The FAD-dependent oxidoreductase from Chaetomium thermophilum (CtFDO) is a novel thermostable glycoprotein from the glucose–methanol–choline (GMC) oxidoreductase superfamily. However, CtFDO shows no activity toward the typical substrates of the family and high-throughput screening with around 1000 compounds did not yield any strongly reacting substrate. The structure of CtFDO reveals an unusually wide-open solvent-accessible active-site pocket with a unique His–Ser amino-acid pair putatively involved in enzyme catalysis. A series of six crystal structures of CtFDO complexes revealed five different subsites for the binding of aryl moieties inside the active-site pocket and conformational flexibility of the interacting amino acids when adapting to a particular ligand.

Cystamine, which was used for CtFDO complex preparation by co-crystallization, was found to improve the diffraction quality of the CtFDOdegl crystal, but without any electron density being found for the compound. The structure is presented as the ligand-free structure of CtFDOdegl and is referred to as the CtFDO:free structure. The CtFDO:free crystal structure has two CtFDOdegl molecules (chains A and B) in the asymmetric unit, with an r.m.s.d. on Cα atoms of 0.12 Å. The cofactor is noncovalently bound to the apo­enzyme via hydrogen bonds to 13 surrounding residues (Ile56, Ser57, Glu77, Ala78, Val124, Gly128, Asn132, Ala133, Val135, Val273, Ile597, Ser607 and Met609) and indirectly via 12 water molecules. A composite OMIT map of the isoalloxazine ring confirms the nonplanar conformation of the ring with a 20.0° (21.4° in chain B) bend around the N5–N10 axis (measured for atoms C4—N5—C6), which indicates the reduced state of the cofactor. Absorption spectra of an unliganded CtFDOdegl crystal measured before and after X-ray exposure showed that FAD was oxidized before and reduced after exposure and that the reduction occurred during X-ray exposure. One exception is His564, which is always modelled in one conformation enforced by the stabilizing hydrogen bond with Gln351. The active-site pocket of CtFDO:free is occupied by water molecules, two of which are in the CS. The first one, the active-site water molecule (WAS), was found bridging four atoms: His564 Nɛ2 (3.0 Å; 3.1 Å in chain B), Ser607 Oγ (‘in’ conformer, 3.1 Å; 2.9 Å in chain B), Asn562 Nδ2 (3.3 Å) and FAD O4 (3.5 Å). The second water molecule, which is more distant from the isoalloxazine ring (WDAS), is bound between WAS (2.4 Å; 2.6 Å in chain B), Asn562 Nδ2 (3.5 Å; 3.4 Å in chain B), FAD O4 (3.6 Å; 3.8 Å in chain B) and Tyr OH (3.5 Å in chain B, 4.7 Å in chain A).

>NVHSNYTFIIAGGGISGLTLADRLTEDPRVTVLVIEAGPLDRGEDGILVPGAFSPWLYFWPGLVSTPQAGLNNRTVDVITAQVVGGGSTINAMVYLRGDKDDYDSWGALGNPGWSWNSMLPYFIKSETFTPPSPELAAAGNITWDGSIRGRSGPVNYSYPNYFFPGSENWWNAANEVGLPPVKDPMAGSKQGVFWIPSAIDARTMTRSHARRNHYDRVSSRPNYHILPSHLVSKILFRGKQAIGVSYIPTSGGNTTTNVYASKEITLAAGGLGTPKILQLSGIGPRKLLNELGIPVISDLPGVGQNLQDQPTLTIPYTFTNNVFPNTDSLTTNATYNAEQRALYDSSKQGAYTIVNSLSTNIGVMSLQRAAPKSYRQIIAAARARSASLSLPPGTDPAVIRGYQAQRNAILKQFENPNVGVGTVHWGTGSSALVYHLKPLSRGTVNIRSTNPLDAPEIDYRTGTDPIDAQVYTSLFRKNREIFNAPSMRVLGPSEAAPFGANLTTDEEIYAVMRELINPSNAHQCCTAAMMPKDMGGVVSSEQKVYGVQGLRVADISFWPFQLSGSPMATAYAGAERLADVIKKEHRLAGAPKSL[2x]> MGHHHHHHGNITLTKRQQEFLLLNGWLQLQCG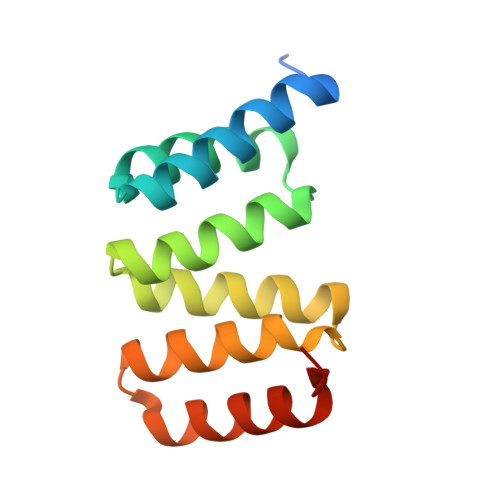HAERACILLDALLTLNPEHLAGRRCRLVALLNNNQGERAEKEAQWLISHDPLQAGNWLCLSRAQQLNGDLDKARHAYQHYLELKDHNESP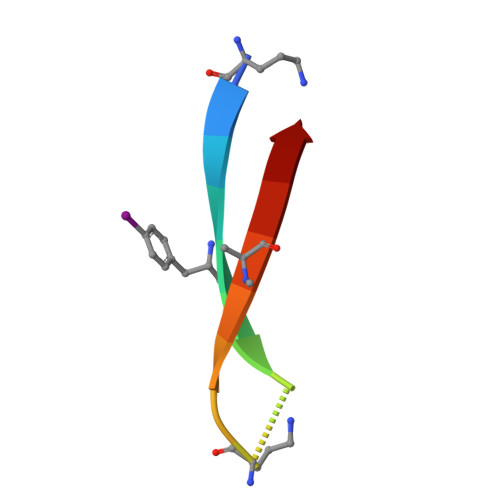> AYLLFYTEAKVAAAVK>[4x]MGHHHHHHAMEGKITPVSVKKVDDKVTLYKTTATADSDKFKISQILTFNFIK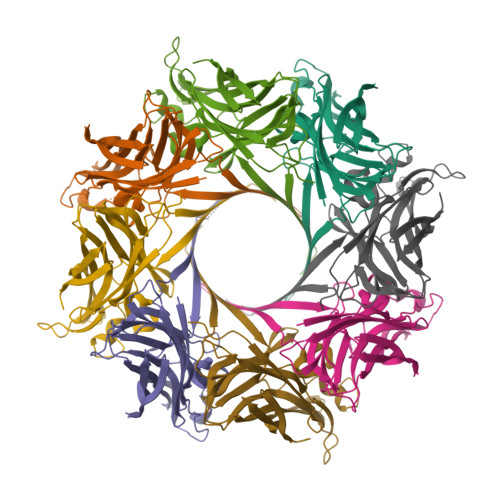DKSYDKDTLVLKATGNINSGFVKPNPNDYDFSKLYWGAKYNVSISSQSNDSVNVVDYAPKNQNEEFQVQNTLGYTFGGDISISNGLSGGLNGNTAFSETINYKQESYRTTLSRNTNYKNVGWGVEAHKIMNNGAGPYGRDSFHPTYGNELFLAGAQSSAYAGQNFIAQHQMPLLSRSNFNPEFLSVLSHRQDGAKKSKITVTYQREMDLYQICWNGFYWAGANYKNFKTRTFKSTYEIDWENHKVKLLDTKETENNK;>[4x]MGHHHHHHAMENKIEDIGQGAEIIKRTQDITSKRLAITQNIQFDFVKDKKYNKDALVVKMQGFISSRTTYSDLKKYPYIKRMIWPFQYNISLKTKDSNVDLINYLPKNKIDSADVSQKLGYNIGGNFQSAPSIGGSGSFNYSKTISYNQKNYVTEVESQNSKGVKWGVKANSFVTPNGQVSAYDQYLFAQDPTGPAARDYFVPDNQLPPLIQSGFNPSFITTLSHERGKGDKSEFEITYGRNMDATYAYVTRHRLAVDRKHDAFKNRNVTVKYEVNWKTHEVKIKSITPK>[4x]SMMNLLRRSGKRRRSESGSDSFSGSGGDSSASPQFLSGSVLSPPPGLGRCLKAAAAGECKPTVPDYERDKLLLANWGLPKAVLEKYHSFGVKKMFEWQAECLLLGQVLEGKNLVYSAPTSAGKTLVAELLILKRVLEMRKKALFILPFVSVAKEKKYYLQSLFQEVGIKVDGYMGSTSPSRHFSSLDIAVCTIERANGLINRLIEENKMDLLGMVVVDELHMLGDSHRGYLLELLLTKICYITRKSASCQADLASSLSNAVQIVGMSATLPNLELVASWLNAELYHTDFRPVPLLESVKVGNSIYDSSMKLVREFEPMLQVKGDEDHVVSLCYETICDNHSVLLFCPSKKWCEKLADIIAREFYNLHHQAEGLVKPSECPPVILEQKELLEVMDQLRRLPSGLDSVLQKTVPWGVAFHHAGLTFEERDIIEGAFRQGLIRVLAATSTLSSGVNLPARRVIIRTPIFGGRPLDILTYKQMVGRAGRKGVDTVGESILICKNSEKSKGIALLQGSLKPVRSCLQRREGEEVTGSMIRAILEIIVGGVASTSQDMHTYAACTFLAASMKEGKQGIQRNQESVQLGAIEACVMWLLENEFIQSTEASDGTEGKVYHPTHLGSATLSSSLSPADTLDIFADLQRAMKGFVLENDLHILYLVTPMFEDWTTIDWYRFFCLWEKLPTSMKRVAELVGVEEGFLARCVKGKVVARTERQHRQMAIHKRFFTSLVLLDLISEVPLREINQKYGCNRGQIQSLQQSAAVYAGMITVFSNRLGWHNMELLLSQFQKRLTFGIQRELCDLVRVSLLNAQRARVLYASGFHTVADLARANIVEVEVILKNAVPFKSARKAVDEEEEAVEERRNMRTIWVTGRKGLTEREAAALIVEEARMILQQDLVEM

DNA polymerase theta (Polθ) has been identified as a crucial alternative non-homologous end-joining factor in mammalian cells. Polθ is distinct among human DNA polymerases, exhibiting not only a C-terminal DNA polymerase domain (Seki et al., 2003, Shima et al., 2003, Yousefzadeh and Wood, 2013) but also an N-terminal domain exhibiting similarity and motifs typical of superfamily 2 (SF2) helicases (Singleton et al., 2007), separated by a long and lesser-conserved central domain of unknown function (Seki et al., 2003, Shima et al., 2003, Yousefzadeh and Wood, 2013) (Singleton et al., 2007). The Polθ helicase domain (Polθ-HLD) is a member of the SF2 helicases, most closely related to the Ski2/Hel308 family of helicases, which are involved in the ATP-dependent 3′-5′ unwinding of lagging strands on replication forks (Tafel et al., 2011, Buttner et al., 2007, Guy and Bolt, 2005), thought to facilitate replication restart at stalled or damaged forks. Like its archaeal homologs, Polθ-HLD comprises five subdomains including the two core helicase domains and three additional, closely associated globular domains.

Using a slightly longer construct (residues 1–894), we obtained crystals of the apo protein, which diffracted to 3.55-Å resolution in a different crystal form containing four copies of Polθ-HLD in the asymmetric unit. Slight differences are seen in the ordering and positioning of various loops that are probably a result of local crystal contacts, as well as minor differences in domain orientation with the nucleotide-bound complexes (discussed later). In the apo crystals, 32 additional residues can be seen at the N terminus. These residues form an extended loop and α-helix (only fully ordered in chain A, due to crystal packing), which packs against the rest of the D1 domain and is unique among the structures of SF2 helicases solved to date. Analysis of the asymmetric unit of the apo crystals reveals four forming a tetrameric clover-shaped molecule with D2 symmetry. Each subunit in the potential tetramer contacts all three of its neighbors, with the interface between chains AC and BD in the apo crystals being slightly more extensive (850-Å2 interface area) and hydrophobic than the interface linking chains AD and BC (600-Å2 interface area), as calculated by the program PISA. Finally, a much smaller interface (180 Å2) that is composed entirely of polar contacts connects AB and CD. The interfaces are almost entirely composed of contacts from the inserted regions of domain 4, explaining why the quaternary structure is not generally conserved across the Hel308 family (archaeal Hel308/Hjm proteins were reported to be monomeric). Furthermore, the fact that the D1 and D2 domains are not constrained by symmetry contacts suggests they would be free to move relative to each other as is required for the helicase mechanism.> MKGFFAGVVAAATLAVASAGDYCGQWDWAKSTNYIVYNNLWNKNAAASGSQCTGVDKISGSTIAWHTSYTWTGGAATEVKSYSNAALVFSKKQIKNIKSIPTKMKYSYSHSSGTFVADVSYDLFTSSTASGSNEYEIMIWLAAYGGAGPISSTGKAIATVTIGSNSFKLYKGPNGSTTVFSFVATKTITNFSADLQKFLSYLTKNQGLPSSQYLITLEAGTEPFVGTNAKMTVSSFSAAVN;> MDQWILGILGFVSTFLCLIGLLLVPVSANIEGDALNALKTNLADPNNVLQSWDPTLVNPCTWFHVTCNSENSVTRVDLGNANLSGQLVPQLGQLPNLQYLELYSNNISGRIPFELGNLTNLVSLDLYLNRLNGPIPDTLG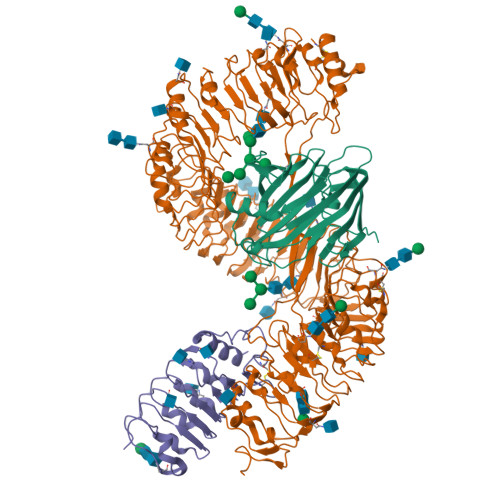KLQKLRFLRLNNNSLNGRIPMLLTTVISLQVLDLSNNNLTGPVPVNGSFSLFTPISFANNPLDIPPAAPPPPISPMPPSSSGVGNSAT;> MGKREYPSSAHFLVTLSLLLLQAAFGLTLCIEKERDALLEFKRGLSDNFGQLSTWGDEEDKKECCKWKGIECNKTTGHVIVLDLHNAFTCSASACFAPRLTGKLSPSLLELEYLNFLDLSVNEFERSEIPRFICSFKRLEYLNLSSSFFSGLIPTQFKNLTSLRILDLGYNNLIVKDLTWLSHLSSLELLSLGGSDFQVKNWFQEITKLPLLKELDLSLCGLSKLVPSPAEIANSSLISLSVLHLCCNEFSSSAKYSWLFNFSTSLTSIDLSNNQLDGQIDDRFGNLMYLEHLNLANELNLKGGIPSSFGNLTRLRYLDMSNTRTYQWLPELFVRLSGSRKTLEVLGLNDNSMFGSLVDVTRFSALKRLYLQKNVLNGFFMERFGQVSSLEYLDLSDNQMRGPLPDLALFPSLRELHLGSNHFNGRIPQGIGKLSQLKILDVSSNRLEGLPESMGQLSNLESFDASYNVLKGTITESHLSNLSSLVDLDLSFNSLALKTSIDWLPPFQLQVINLPSCNLGPSFPKWLQSQNNYTVLDISLANISDALPSWFSGLPPDIKILNLSNNQISGRVSDLIENAYDYMVIDLSSNNFSGPLPLVPTNVQIFYLHKNQFFGSISSICKSTTGATSLDLSHNQFSGELPDCWMNATNLAVLNLAYNNFSGKLPQSLGSLTNLEALYMRQNSFSGMLPSLSQCQSLQILDLGGNKLTGRIPAWIGTDLLNLRILSLRFNKFYGSISPIICQLQFLQILDLSANGLAGKIPQCFNNFTLLHQENGLGEPMEFLVQGFYGKYPRHYSYLGNLLVQWKNQEAEYKNPLTYLKTIDLSSNKLVGGIPKEMAEMRGLKSLNLSRNDLNGSIIKGIGQMKMLESLDLSRNQLSGMIPKDLANLTFIGVLDLSNNHLSGRIPSSTQLQTFERSSYSGNAQLCGPPLQEC>MKLTPKELDKLMLHYAGELAKKRKEKGIKLNYVEAVALISAHIMEEARAGKKTAAELMQEGRTLLKPDDVMDGVASMIHEVGIEAMFPDGTKLVTVHTPIEANGKLVPGELFLKNEDITINEGKKAVSVKVKNVGDRPVQIGSHFHFFEVNRCLDFDREKTFGKRLDIASGTAVRFEPGEEKSVELIDIGGNRRIFGFNALVDRQADNESKKIALHRAKERGFHGAKSDDNYVKTIKE[12x];>[12x]MKKISRKEYVSMYGPTTGDKVRLGDTDLIAEVEHDYTIYGEELKFGGGKTLREGMSQSNNPSKEELDLIITNALIVDYTGIYKADIGIKDGKIAGIGKGGNKDMQDGVKNNLSVGPATEALAGEGLIVTAGGIDTHIHFISPQQIPTAFASGVTTMIGGGTGPADGTNATTITPGRRNLKWMLRAAEEYSMNLGFLAKGNASNDASLADQIEAGAIGFKIHEDWGTTPSAINHALDVADKYDVQVAIHTDTLNEAGCVEDTMAAIAGRTMHTFHTEGAGGGHAPDIIKVAGEHNILPASTNPTIPFTVNTEAEHMDMLMVCHHLDKSIKEDVQFADSRIRPQTIAAEDTLHDMGIFSITSSDSQAMGRVGEVITRTWQTADKNKKEFGRLKEEKGDNDNFRIKRYLSKYTINPAIAHGISEYVGSVEVGKVADLVLWSPAFFGVKPNMII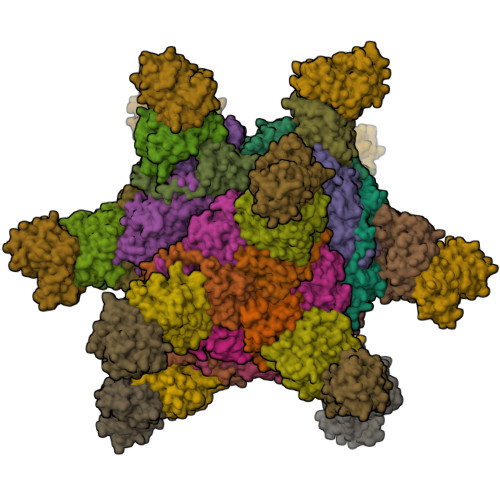KGGFIALSQMGDANASIPTPQPVYYREMFAHHGKAKYDANITFVSQAAYDKGIKEELGLERQVLPVKNCRNITKKDMQFNDTTAHIEVNPETYHVFVDGKEVTSKPANKVSLAQLFSIF;>MNTYAQESKLRLKTKIGADGRCVIEDNFFTPPFKLMAPFYPKDDLAEIMLLAVSPGMMRGDAQDVQLNIGPNCKLRITSQSFEKIHNTEDGFASRDMHIVVGENAFLDFAPFPLIPFENAHFKGNTTISLRSSSQLLYSAIIVAGRVARNELFKFNRLHTKISILQDEKPIYYDNTILDPKTTDLNNMCMFDGYTHYLNLVLVNCPIELSGVRECIEESEGVDGAVSETASSHLCVKALAKGSEPLLHLREKIARLVTQTTTQKVWSHPQFEK[12x];>MDKGKSVKSTEKSVGMPPKTPKTDNNAHVDNEFLILQVNDAVFPIGSYTHSFGLETYIQQKKVTNKESALEYLKANLSSQFLYTEMLSLKLTYESALQQDLKKILGVEEVIMLSTSPMELRLANQKLGNRFIKTLQAMNELDMGEFFNAYAQKTKDPTHATSYGVFAASLGIELKKALAHYLDAQTSNMVINCVKSVPLSQNDGQKILLSLQSPFNQLIEKTLELDESHLCTASVQNDIKAMQHESLYSRLYMS[12x]> GMTILSDVAALGQQIWLDNLSRSLVQSGELAQMLKQGVCGVTSNPAIFQKAFAGDALYADEVAALKRQNLSPKQRYETMAVADVRAACDVCLAEHESTGGKTGFVSLEVSPELAKDAQGTVEEARRLHAAIARKNAMIKVPATDAGIDALETLVSDGISVNLTLLFSRAQTLKAYAAYARGIAKRLAAGQSVAHIQVVASFFISRVDSALDATLPDRLKGKTAIALAKAAYQDWEQYFTAPEFA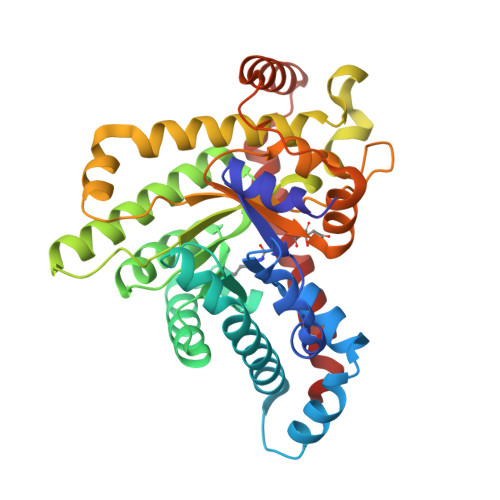ALEAQGANRVQLLWASTGVKNPAYPDTLYVDSLIGVHTVNTVPDATLKAFIDHGTAKATLTESADEARARLAEIAALGIDVETLAARLQEDGLKQFEEAFEKLLAPLV>GAMAQNITARIGEPLVLKCKGAPKKPPQRLEWKLNTGRTEAWKVLSPQGGGPWDSVARVLPNGSLFLPAVGIQDEGIFRCQAMNRNGKETKSNYRVRVYQIPGKPEIVDSASELTAGVPNKVGTCVSEGSYPAGTL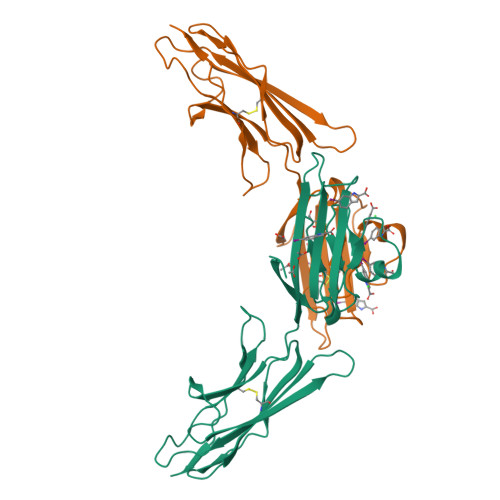SWHLDGKPLVPNEKGVSVKEQTRRHPETGLFTLQSELMVTPARGGDPRPTFSCSFSPGLPRHRALRTAPIQPRVWE[2x]> NTEAKPKIDKDFKGKANPDTPRVDKDTPVNHQVGDVVEYEIVTKIPALANYATANWSDRMTEGLAFNKGTVKVTVDDVALEAGDYALTEVATGFDLKLTDAGLAKVNDQNAEKTVKITYSATLNDKAIVEVPESNDVTFNYGNNPDHGNTPKPNKPNENGDLTLTKTWVDATGAPIPAGAEATFDLVNAQAGKVVQTVTLTTDKNTVTVNGLDKNTEYKFVERSIKGYSADYQEITTAGEIAVKNWKDENPKPLDPTEPKVVTYGKKFVKVNDKDNRLAGAEFVIANADNAGQYLARKADKVSQEEKQLVVTTKDALDRAVAAYNALTAQQQTQQEKEKVDKAQAAYNAAVIAANNAFEWVADKDNENVVKLVSDAQGRFEITGLLAGTYYLEE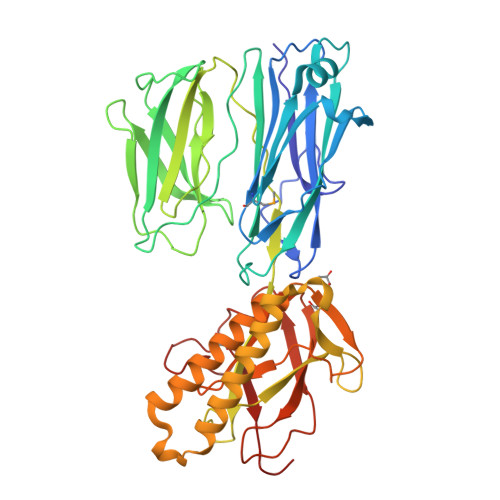TKQPAGYALLTSRQKFEVTATSYSATGQGIEYTAGSGKDDATKVVNKKIT>[2x]MDEFYISIETVGNNIVER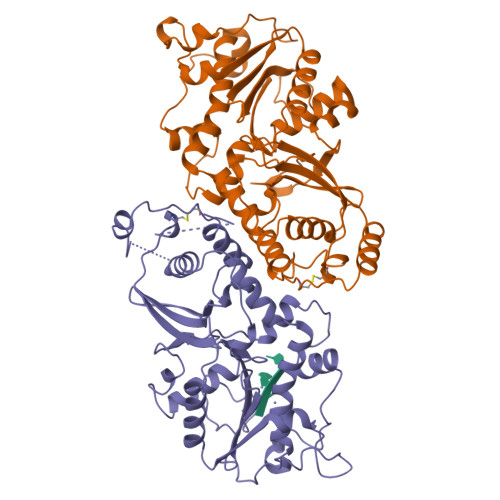YIDENGKERTREVEYLPTMFRHCKEESKYKDIYGKNCAPQKFPSMKDARDWMKRMEDIGLEALGMNDFKLAYISDTYGSEIVYDRKFVRVANCDIEVTGDKFPDPMKAEYEIDAITHYDSIDDRFYVFDLLNSMYGSVSKWDAKLAAKLDCEGGDEVPQEILDRVIYMPFDNERDMLMEYINLWEQKRPAIFTGWNIEGFDVPYIMNRVKMILGERSMKRFSPIGRVKSKLLQNMYGSKEIYSIDGVSILDYLDLYKKFAFTNLPSFSLESVAQHETKKGKLPYDGPINKLRETNHQRYISYNIIDVESVQAIDKIRGFIDLVLSMSYYAKMPFSGVMSPIKTWDAIIFNSLKGEHKVIPQQGSHVKQSF9-{5-O-[(S)-hydroxy(phosphonooxy)phosphoryl]-alpha-D-ribofuranosyl}-N-(prop-2-yn-1-yl)-9H-purin-6-amine 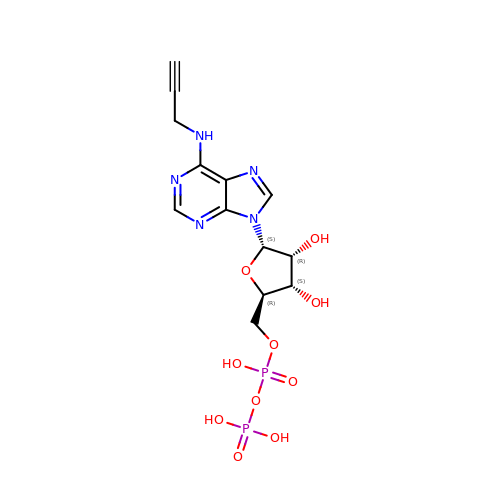| C13 H17 N5 O10 P2 | DYWGWOPDXRINLT-HMMKDHSLSA-N>AFMSQMMQMYQQVGPAQFSAMIGQFAPYFASIAPQFVELRPGYAEVTFPKRREVLNHIGTVHAIALCNAAELAAGTMTDASIPAGHRWIPRGMTVEYLAKATGDVRAVADGSQIDWQATGNLVVPVVAYVDDKPVFRAEITMYVS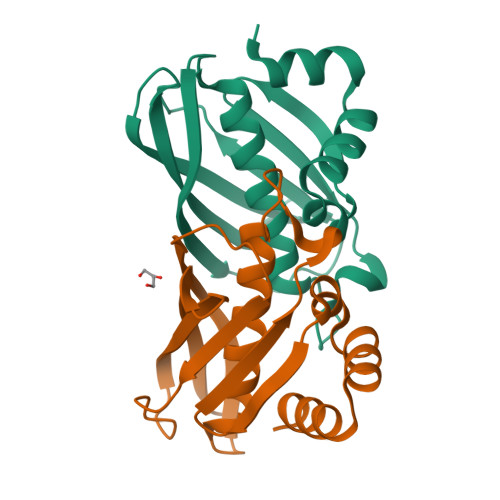QA[2x]> AMSNNKIKRKDASPEQEAIESFTSLTKCDPKVSRKYLQRNHWNINYALNDYYDKEIGTFTDEVSTVAHPPVYPKELTQVFEHYINNNLFDIDSLVKFIEELGYNLEDLATLCLAHLLGYKKLEEPLKREDFLSTWFMQGCSTISDMQECIKTLDVKLHEDLQYFTQIYNYAFNLILDPNRKDIDTDEGIQYWKLFFQPEYPVRMEPDLLEAWFRFLRDEGKTTISKDTWRMLLLFFKRYPTIQKII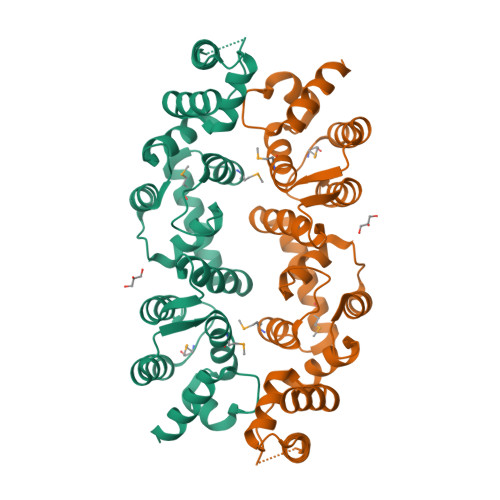SDYDETAAWPFIIDEFYECLQDQQ>[4x]MATRSPGVVISDDEPGYD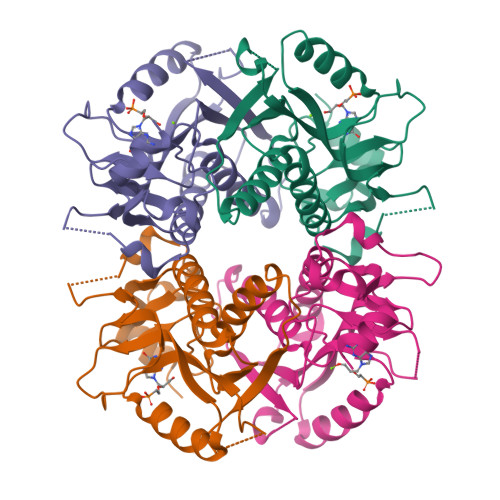LDLFAIPNHYAEDLERVFIPHGLIMDRTERLARDVMKEMGGHHIVALCVLKGGYKFFADLLDYIKALNRNSDRSIPMTVDFIRLKSYANDQSTGDIKVIGGDDLSTLTGKNVLIVEDIIDTGKTMQTLLSLVRQYNPKMVKVASLLVKRTPRSVGYKPDFVGFEIPDKFVVGYALDYNEYFRDLNHVAVISETGKAKYKA>AKEWQENKSWNAHFTEHKSQGVVVLWNENKQQGFTNNLKRANQAFLPASTFKIPNSLIALDLGVVKDEHQVFKWDGQTRDIATWNRDHNLITAMKYSVVPVYQEFARQIGEARMSKMLHAFDYGNEDISGNVDSFWLDGGIRISATEQISFLRKLYHNKLHVSERSQRIVKQAMLTEANGDYIIRA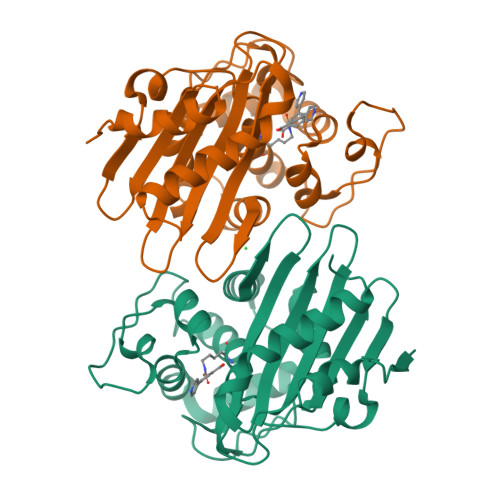KTGYSTRIEPKIGWWVGWVELDDNVWFFAMNMDMPTSDGLGLRQAITKEVLKQEKIIP[4x]> MPWEDYVGKTLPVGSRLPPNFKTYDYFDRATGAVVSAKSLDTQTMAKLSNPNQVYSSIKKNIDVTAKFEKASLSGVT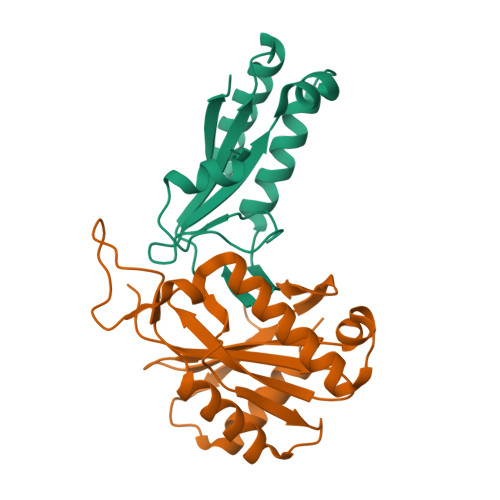VNSSMITSKEVRLAVPVNTTKAQWTEINRAIEYGKNQGVKVTVTQVK;> MNDIVKSAWASVKMNTDFICVDTYSGYRSNQLDPLGVQHLSSPDVSDLDLGEMVKDALSHSRFVLPAPRTDIWIHPEVTFDLDLYDSRRTVERYDEWVKKLMVHYGYKTKRALFKDMKSCDICCNHDAITISPTRHEKLEVWGGTGLKGSDNVILSVDSSPTEIGAGLRLALSRCKGLEHHHHHH>[4x]GSHMATFQTDADFLLVGDDTSRYEEVMKTFDTVEAVRKSDLDDRV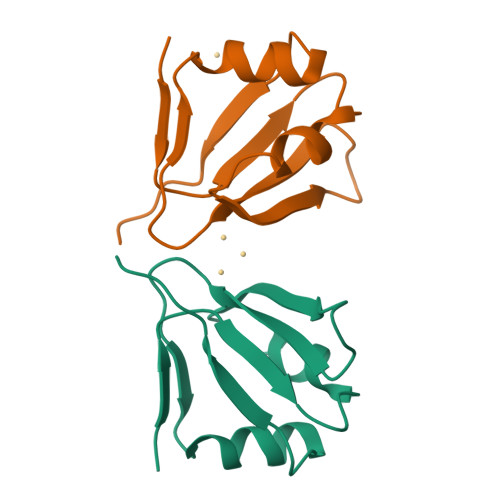YMVCLKQGSTFVLNGGIEELRLLTGDSTLEIQPMIVPTTE> MGRVADTIARGPSNSEQIPALTAVETGHTSQVDPSDTMQTRHVHNYHSRSESSIENFLCRSACVIYIKYSSAESNNLKRYAEWVINTRQVAQLRRKMEMFTYIRCDMELTFVITSHQEMSTATNSDVPVQTHQIMYVPPGGPVPTSVNDYVWQTSTNPSIFWTEGNAPPRMSIPFMSIGNAYTMFYDGWSNFSRDGIYGYNSLNNMGTIYARHVNDSSPGGLTSTIRIYFKPKHVKAYVPRPPRLCQYKKAKNVNFDVEAVTTERASLVTT;> SDRVRSITLGNSTITTQECANVVVGYGVWPDYLSDEEATAEDQPTQPDVATCRFYTLNSVKWEMQSAGWWWKFPDALSEMGLFGQNMQYHYLGRSGYTIHVQCNASKFHQGCLLVVCVPEAEMGCTNAENAPTYGDLCGGETAKQFEQNAVTGETAVQTAVCNAGMGVGVGNLTIYPHQWINLRTNNSATIVMPYINSVPMDNMFRHNNFTLMIIPFAPLDYVTGASSYIPITVTVAPMSAEYNGLRLAGHQ;> GLPTMLTPGSTQFLTSDDFQSPSAMPQFDVTPEMNIPGQVRNLMEIAEVDSVVPINNLQANLKTMEAYRVQVRSTDEMGGQIFGFPLQPGASSVLQRTLLGEILNYYTHWSGSLKLTFVFCGSAMATGKFLLAYSPPGAGAPDSRKNAMLGTHVIWDVGLQSSCVLCVPWISQTHYRYVVDDKYTASGFISCWYQTNVIVPAEAQKSCYIMCFVSACNDFSVRMLRDTQFIKQDTFYQ;> MGAQVSTQKTGAHETSLSASGNSIIHYTNINYYKDAASNSANRQDFTQDPSKFTEPVKDVMIKSLPALN

The protomers assemble to form the ∼30 nm wide icosahedral shell with a pseudo T = 3 arrangement that encapsidates the linear single-stranded RNA genome. The arrangement occurs because of the similar structures of VP1, VP2, and VP3, which all adopt an eight-stranded, antiparallel β-barrel fold despite having low sequence homology. Recently, we discovered a second druggable pocket at a conserved VP1–VP3 interprotomer interface in the viral capsid. Here, in an effort to better understand the druggable features of the interprotomer pocket, we have analyzed high-resolution structures of two medically important enteroviruses, coxsackieviruses B3 and B4, complexed with interprotomer-targeting compounds CP17 and CP48, respectively.

We chose to work with CVB4 because no structure exists for this important human pathogen. The outer surface of the virus particle is similar to that of other enteroviral capsids, with major features including the fivefold star-shaped mesas, threefold propeller-like protrusions, and twofold depressions. The control structure of CVB4 incubated without compound revealed no additional density inside the pocket. We did not detect a conformational change induced by the presence of CP48 (RMSD for native versus CP48-bound virus: 0.45 Å). First, in CP48–CVB4, density corresponding to the native pocket factor within the β-barrel of VP1 appears to be altered by the presence of drug; however, there were no major conformational changes in the four capsid proteins based on comparison to the control structure of CVB4 alone. Another difference between CVB4 and CVB3 occurs in the exposed loop linking β-strands B and C of VP1, which for CVB4 differs in length and conformation. We were unable to perform similar experiments with CVB4 here because there is no infectious clone available.> MLKQVEIFTDGSCLGNPGPGGYGAILRYRGREKTFSAGYTRTTNNRMELMAIIVALEALKEHCEVILSTDSQYVRQGITQWIHNWKKRGWKTADKKPVKN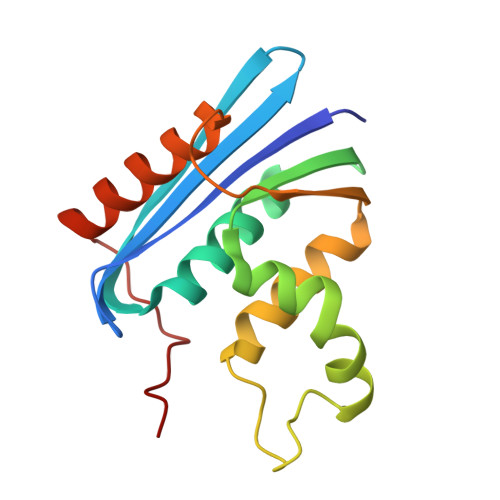VDLWQRLDAALGQHQIKWEWVKGHAGHPENERCDELARAAAMNPTLEDTGYQVEV> LVPRGSHMLFQNVSIAGLAHIDAPHTLTSKEINERLQPTYDRLGIKTDVLGDVAGIHARRLWDQDVQASDAATQAARKALIDANIGIEKIGLLINTSVSRDYLEPSTASIVSGNLGVSDHCMTFDVANACLAFINGMDIAARMLERGEIDYALVVDGETANLVYEKTLERMTSPDVTEEEFRNELAALTLGCGAAAMVMARSELVPDAPRYKGGVTRSATEWNKLCRGNLDRMVTDTRLLLIEGIKLAQKTFVAAKQVLGWAVEELDQFVIHQVSRPHTAAFVKSFGIDPAKVMT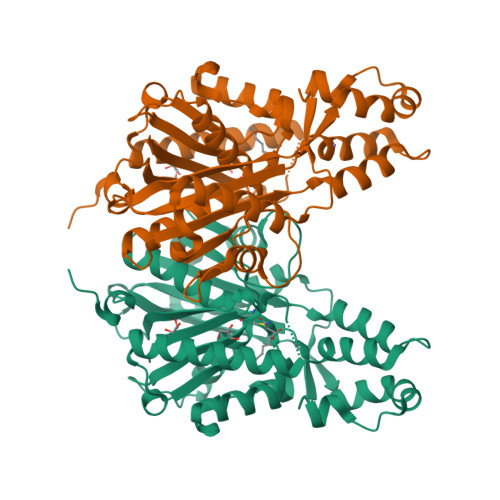IFGEHGNIGPASVPIVLSKLKELGRLKKGDRIALLGIGSGLNCSMAEVVW> GPGS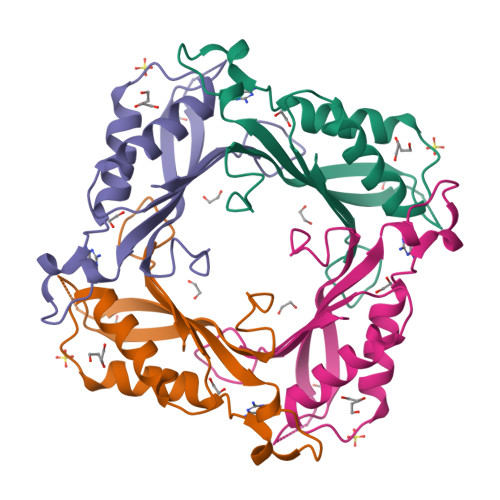MTGTTMFAALLHPRLADCRRLYLRNHEVYMNIGAFEHEKRGEQRVVINVDLFVPLALTTPVEDKLREVVDYDLMKQSVAQCVARGHIHLQETLCDAIAASLLAHDAVRAVRVSTEKPDAYPDCDAVGVEVFRIKDEERA>[2x]GMQQPTASVVSYVAEYHKATETTMGRYKKVIEITGHDEVAAKLLEGLIDAGTRYFSKVVEMEHRMASARFRLDGEELRELTETL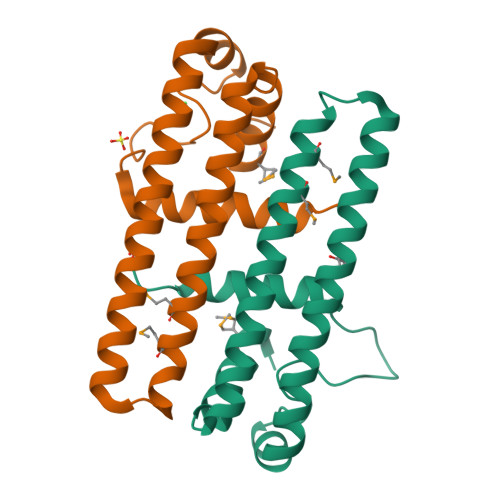DRSRRLAHESLISSLHVFNRYIVKEYGEELKEAGIEGGIFPKPEANRDRIAIADWAGELLTGIYENRHR>GPLGSMEGLFSQKSFLVLGFSVENKCNIVDIIREHAGKIVSLPSRIVADYAVVPLLGCEVDVTVGEVVTNTWLVTCIDNQTLVDPKSNPLFTPVSVMSGVTPLEDCVISFSQCVGAERDSLVFLANHLGASVQEFFVRKANAKKGMLASTHLIVKEPTGSKYEAAKKWSLPAVNI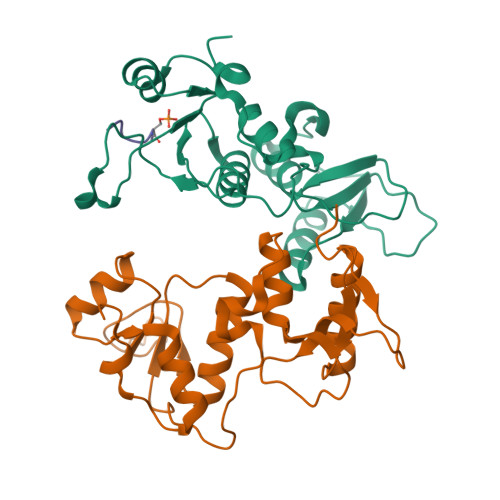SWLLETARIGKRADENHFLVDNAPK[8x];>DTDFVPPSPEEII[4x]>SNAMRRVEKVIIVEGRSDKQKVAAVLNEPVVIVCTNGTISDARLEELADELEGYDVYLLADADEAGEKLRRQFRRMFPEAEHLYIDRAYREVAAAPIWHLAQVLLRARFDVRIESLMRGR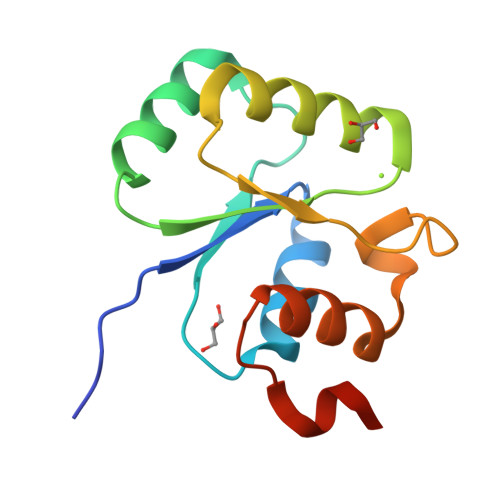GE[3x]DOUBLY FUNCTIONALIZED 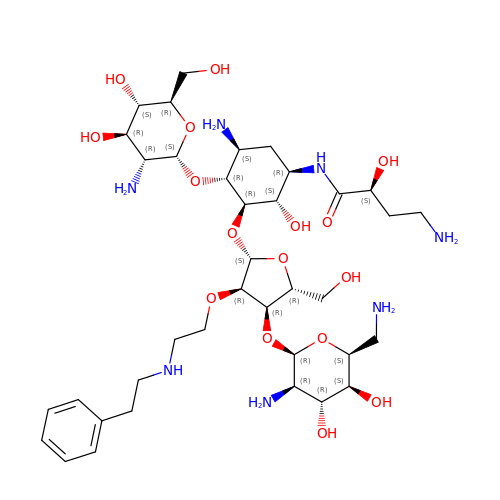PAROMOMYCIN PM-II-162 | C37 H65 N7 O16 | KITFYJSEQIOMTC-AFTVZRPJSA-N> SDMKKNIVQWNSRYSYNQLKNKDSLIMFLVEIFRSLFVSNCIDKNIDNVLLSIEEMFIDHYYNPQHSRLKYLIDDVGIFFTKLPITKAFHTYNKKYRITKRLYAPPTFNEVRHILNLAQILSLEEGLDLLTFDANETLYPDGHDFNDEVLASYISCLLKKMNIAIVTAASYNNDAEKYQKRLENLLKYFSKHNIKDGSYKNFYVMGGESNYL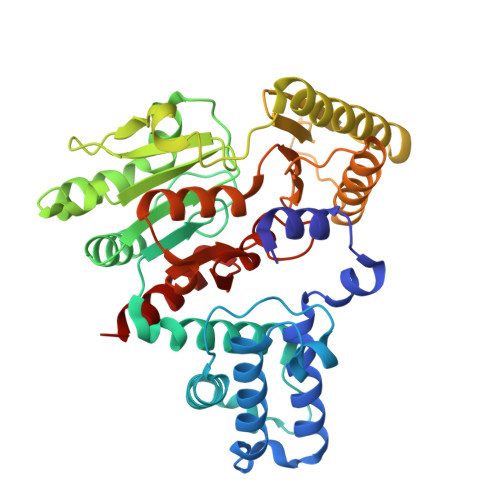FKCNEEATLYSVPENEWRHYKKFVDYDTVQEILNISEKCLEKVIKDFGLCAQIQRKEKSIGLVPNKIPSLNIKNEQKNYMIKYEVLEEAVIRIKKEIIKNKITAPYCAFNGGQDLWVDVGNKAEGLLILQKLLKIQKKKCCHIGDQFLHSGNDFPTRFCSLTLWVSNPQETKACLKSIMHLN Here, we reveal the extended and contracted atomic structures of an intact contractile-tailed phage (φCD508) that binds to and penetrates the protective S-layer of the Gram-positive human pathogen Clostridioides difficile. The virion can be divided into five distinct regions: the head, neck, tail, baseplate, and needle. Structures of purified φCD508 virions in both extended and contracted conformations were determined by single-particle EM of frozen-hydrated samples; the resolution ranged from 2.6 to 4.0 Å for the extended phage, and 2.9 to 4.2 Å for the contracted form.

The neck links the capsid to the tail. The portal in turn connects to the neck, which is made up of three protein complexes with a VIRFAM type I neck arrangement, comprising one dodecameric ring (gp50) and two hexameric rings (gp51 and gp53). The symmetry is therefore reduced from 12-fold down to 6-fold, traveling down the neck. The first complex in the neck is the head-to-tail adaptor gp50, which assembles into a 12-fold symmetric ring and acts to resolve a symmetry mismatch between the portal and the tail. The neck valve protein gp51 forms a hexameric complex and represents the narrowest constriction in the neck lumen, ∼23 Å in diameter at its minimum. gp51 has structural homology to the “stopper” protein of SPP1, which is proposed to prevent DNA leakage from the capsid (RMSD ∼8 Å for 53 out of 80 Cɑ pairs). In our structure, strong density in the lumen of the channel weakens around the neck valve, suggesting the neck valve may also constitute the point at which DNA is prevented from exiting through the tail of the φCD508 before contraction. Below the constriction, a weaker density is present, which likely constitutes the tape measure protein gp59, although the enforced sixfold symmetry in the reconstruction prevents identification or building of a model into this region.

>MYNDDYIEEASFLNGSDVVILIDGVEELYMEEIKADFEQDEQSIKLLGCQNEISRVGTTKGSFSLNGYKTDSKFAKLGFRSFEIIYNLSNSETLGYESIRLKNCRLKKLPLINSKAGEIVKIEVEGSFRGYDLLNEL[6x];>MINIDRRRKDIIRTININPTNITITSIKKTEIDGAFEETETEIKCVVRIFNEKTAEKQISSEKQGTFSSIRTYGMLVSNDVILEVNSRDSLEFECIYGRMKIVNIYPQIVKGELCGYQCSLERID[6x];>MRAGIRKALIDNIKELKGCYEPNVPNKDTKKPYMVVVQGQDNDHGETIGFERSIEVWIYEGRTTFKKLDKLTKQVVEVLDMNTIVDESENEAFTCIYKGTSENDIVVEEWDAIARGIRFSVIALEDKEDTTNDRWVEALSRHTKDLLEIESYKDNWKKNFIAPCALWRTTHIENKRINYHLIEITKTMKCHVVSKNKDEIVKLLETLETSLIIDKRVRLREDKNMYLTLVSVVEDRESDMFTTGQLTAVFKMIGKIKREGPTMDKIYGNGNLK[6x];>MTPARDLIEKLRLLLNDKDKKSFTDEELNLFLEEADCIYCAASQGWILKSLQYENTVGEMYEYKVGQETYKSSSIKDLVSVAYQNADKFKDMCTNKKEKGSFMLGISTEFEI[12x];>[6x]MATGTWNEKERKEIPGFYNRFKTQAEKSTNTGLKGRLAMPIRANWGDVGKVVTIKNDLRQLKNLFGDDMNYSAFKLGKLALLGNVKELLLYRLVDGNQKKGTLTLKDTTENSAKDVIKLETKYPTARNFNVTIKSNLVDSDKKDFIFFENTKQLFSSSIKGTIDEIVLEINSNLDNEYVIATKVADSDTILANVVNQALEGGNDGCTSITNESYLKALEEFERYSFDSFVLDGVADEALQETTKAWVAKNKELGKDILLFLGGKTEDNIKQINDKSKSFNDENIVNVGSSAYYENIKYTPSEVAVYIAALSVSKGITGSICNAKTIFEEVEPRLSQSEVKECLKSGTLVLDFDDGDVIIVDDVNTFKKYVDDKNEAMGYISNIMFINTINKDTSLKRKEFVGKIFNDATGQTTVICALKKYFEELMSQGIISEFNVDIDTELQATAKADEFYWKWDAVKVDVMKKIYGTGYLG;>[12x]MGIISYVKKLFKRPAGEIMRMSSGNIGVYKLDDSRVDYELARELYQNKNANYKLGSSFVRPIVNSTTGFMGVPHFQIEDEEAQYILDEFVLDNTSKMLKTHTDSLKQGDCYIWITREERENPLYPDKKVRLIYNFISPEEVKEIILDPTTKEPIAYILESQNEWTDLGENKRKAKVKQIITAESRFVEVEGDKIEGLEEGETPNVWGFIPIIHFKNEADETLKYGQSDIEPIEPLLKAYHDVMLHALKGSKMHSTPKLKLKLTDVASFLAHNFGVEDPVKFAKEGGKINLDGHEILFLNKDEEAEFVEVKSAIGDAKELLKLLFYCIVDVSETPEFIFGVHTPSALASVKEQMPIMVNKIRRKREQFTNSWQLLARMVLIMSSNSSGMKYSSYDVTIGWDEVNPRDDKELAETLEKVCCALDKALEGGFISEESTVNFLAQYIDTMSNYISDDPEREGEREKIIKTKMLKYRLDDSQGLNDESNEIEKEINKIKDNNGNG> GTGTA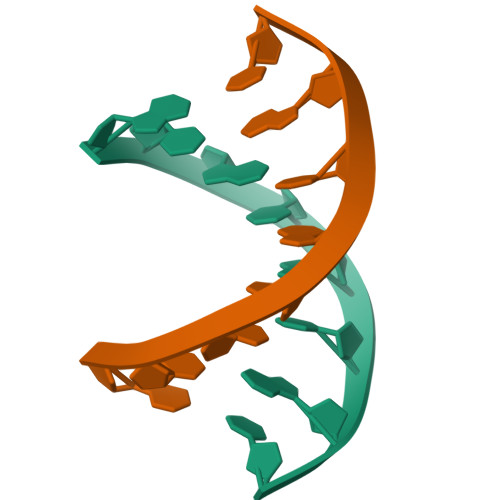CAC> GPGSEF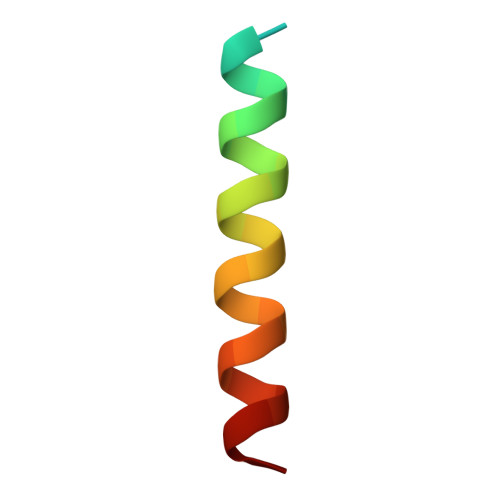SATRELDELMASLSDFKFMAQG>[8x]MGSSHHHHHHAAPLPELLSNNGKHALMVDGAPYIILGSQTNNSSNYPDALKDVWPSMEKMGANTLSIPVAWEQIEPVEGQFDFSFVDVLLKEARQRKVRLVLLWFATWKNNAPHYAPAWVKLDNARFPRVVKEDGDTLNSLSPLGQNTLAADKKAFVELMKYLAKRDKDHTVIMVQVQNEVGTYGAVRDYSPMAQAVFNAAVPDDLIQKLQLKPGTWSQVFGRDADEFFHAYQIARYCDEVTVAGKAIKNLPMYVNVALRNPFNPGLPGQYSSGGGTDNVLHIWKAAAPNIDLIAPDIYFRDYKTVSKVLELYTRPDNALFVAEIGNDQPFARYLFPTLGKGGIGFSPFGMDDTDYTNYPLGAKVYNDETIEQFAQVYRLVNPMMREWARLSYQGQVWGVAEPLDSTTETQKIWNAEATPEEKEQHKKDRASALTQQLDLGLWDAEVTYGRPMFWVTPPEGNTPAAGGALIAQLDDNEYLVTAYKARVEFKPSQELAGKKFMIERVEEGRFEKGKWVMERVWNGDQTDWGLNFTDRPHLLRVKMASYSVQ

GM1-Gangliosidosis and Morquio B disease are two manifestations of mutations on the GLB1 gene that encodes the vital lysosomal β-galactosidase. This enzyme is responsible for removal of a β-galactosyl residue from the non-reducing end of its substrate, converting gangliosides GM1 and GA1 into GM2 and GA2, respectively. Based on X-ray crystallographic studies of compounds 1, 14, 16, 17 as well as 22 and 31 in complex with Cellvibrio japonicus β-galactosidase (CjGH35), a tractable bacterial model which shows around 27% sequence identity with the human enzyme, notably conserved active centers, intensities of inhibition and chaperoning properties, may be partially rationalized. For the inhibitors studied here, the ligand sugar moieties have clear density in all the active sites and overlay with ring C atoms 2 to 5 in similar positions.

In particular, the β-d-galacto configured cyclopentylamine bearing a 4-bromobenzyl moiety at the nitrogen (15), has been found to excel in terms of inhibitory activity and recently prepared compounds 16 and 17 are powerful inhibitors of human lysosomal β-galactosidase and potent pharmacological chaperones for the R201C mutant of this enzyme. For all the C-1-substituents in 1, 16, 17 and 31, (an NH-octyl group in 1 and 16, and NH-C6-NH-dansyl groups in 17 and 31), and the C-5a-substituted NH-C6-NH-dansyl groups in 14 and 22, there are very few interactions between the protein and substituted derivative moieties. The most salient variation in hydrogen bonding occurs at the 2-OH group, which is present in 1, 16 and 17. The group is tethered by interactions with ND2 Asn204 (all 2.8–3.0 Å) and to both OE atoms of Glu349 (2.6–2.7 Å) Hydrogen bonding patterns for 16 and 17 are very similar, despite the different groups bound at C-1, which are probably flexible and show few polar interactions with the protein, and not surprisingly, the Ki values determined for these inhibitors with recombinant human lysosomal β-Gal are very similar. Another key ligand-protein interaction is displayed for compounds 1, 16, 17 and 31, which feature hydrogen bonding interactions from their amine groups at ring position 1 to Glu205 (2.6–2.8 Å) and with a water which is also hydrogen bonded to ND2 Asn135, and in the case of 1, to the C-4 hydroxyl group.>MKKIKPHGPLPSQTQLAYLGDELAAFIHFGPNTFYDQEWGTGQEDPERFNPSQLDAREWVRVLKETGFKKLILVVKHHDGFVLYPTAHTDYSVKVSPWRRGKGDLLLEVSQAATEFDMDMGVYLSPWDAHSPLYHVDREADYNAYYLAQLKEILSNPNYGNAGKFAEVWMDGARGEGAQKVNYEFEKWFETIRDLQGDCLIFSTEGTSIRWIGNERGYAGDPLWQKVNPDKLGTEAELNYLQHGDPSGTIFSIGEADVSIRPGWFYHEDQDPKSLEELVEIYFHSVGRGTPLLLNIPPNQAGLFDAKDIERLYEFATYRNELYKEDLALGAEVSGPALSADFACRHLTDGLETSSWASDADLPIQLELDLGSPKTFDVIELREDLKLGQRIAAFHVQVEVDGVWQEFGSGHTVGYKRLLRGAVVEAQKIRVVITESQALPLLTKISLYKTP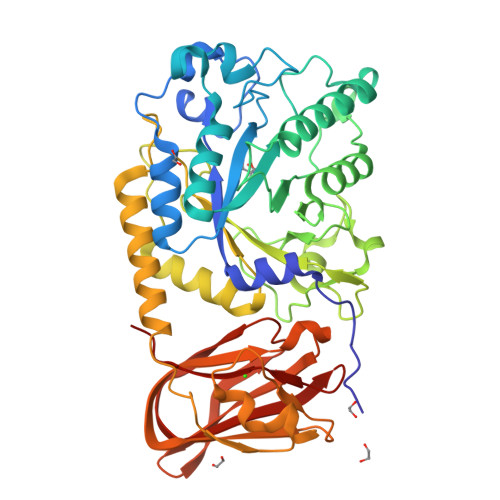G[2x]(1r,4r)-N-methyl-4-(trifluoromethyl)cyclohexan-1-amine 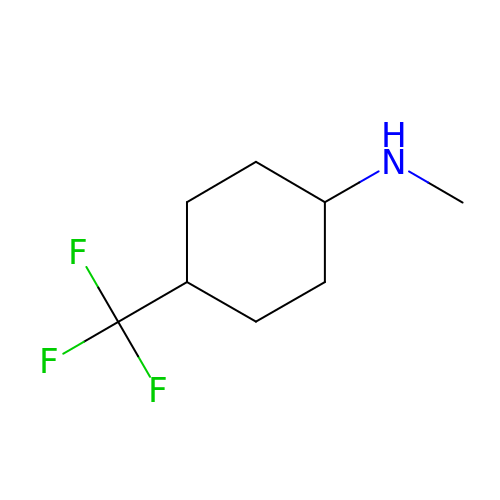| C8 H14 F3 N | QUUODNYZDCDMHQ-LJGSYFOKSA-N> GPLGSATITQDTPINQIFTDTALAEKMKTVLGKTNVTDTVSQTDLDQVTTLQADRLGIKSIDGVEYLNNLTQINFSNNQLTDITPLKNLTKLVDILMNNNQIADITPLANLTNLTGLTLFNNQITDIDPLKNLTNLNRLELSSNTISDISALSGLTSLQQ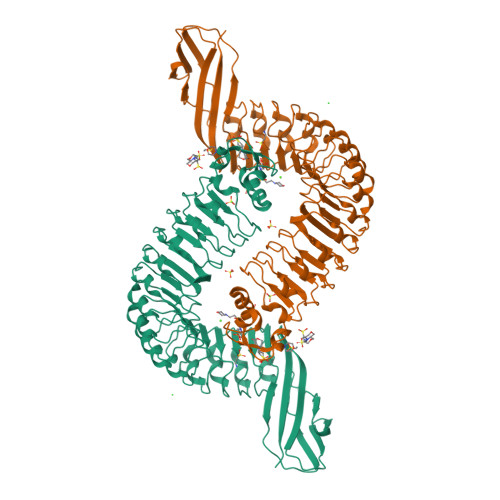LSFGNQVTDLKPLANLTTLERLDISSNKVSDISVLAKLTNLESLIATNNQISDITPLGILTNLDELSLNGNQLKDIGTLASLTNLTDLDLANNQISNLAPLSGLTKLTELKLGANQISNISPLAGLTALTNLELNENQLEDISPISNLKNLTYLTLYFNNISDISPVSSLTKLQRLFFYNNKVSDVSSLANLTNINWLSAGHNQISDLTPLANLTRITQLGLNDQAWTNAPVNYKANVSIPNTVKNVTGALIAPATISDGGSYTEPDITWNLPSYTNEVSYTFSQPVTIGKGTTTFSGTVTQPLKA> MERNKLARQIIDTCLEMTRL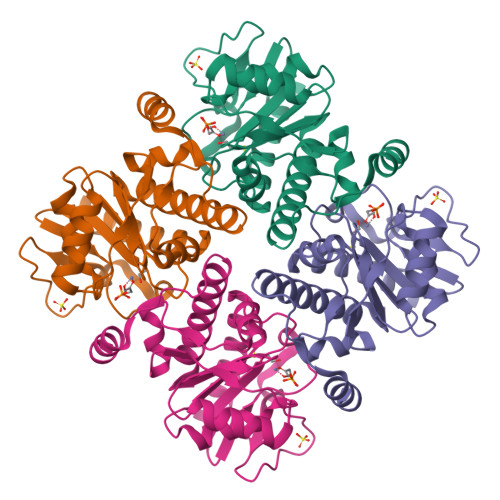GLNQGTAGNVSVRYQDGMLITPTGIPYEKLTESHIVFIDGNGKHEEGKLPSSQWRFHMAAYQSRPDANAVVHNHAVHCTAVSILNRSIPAIHYMIAAAGGNSIPCAPYATFGTRELSEHVALALKNRKATLLQHHGLIACEVNLEKALWLAHEVEVLAQLYLTTLAITDPVPVLSDEEIAVVLEKFKTYGLRIEE>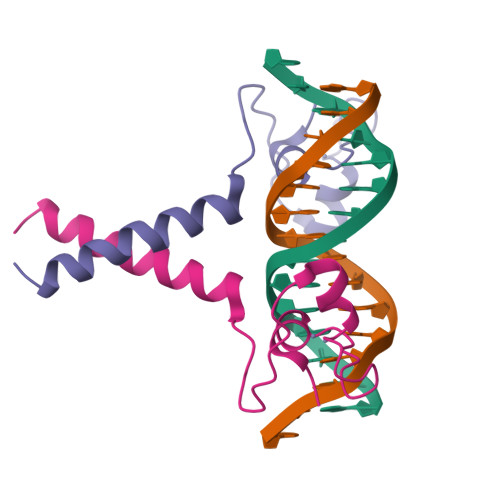KRKFACVECRQQKSKCDACERAPEPCTKCAKKNVPCILKRDFRRTYKRARNEAIEKRFKELTRTLTNLTSDE[2x]> EPVKFKDCGSWVGVIKEVNVSPCPTQPCKLHRGQSYSVNVTFTSNTQSQSSKAVVHGIVMGIPVPFPIPESDGCKSGIRCPIEKDKTYNYVNKLPVKNEYPSIKVVV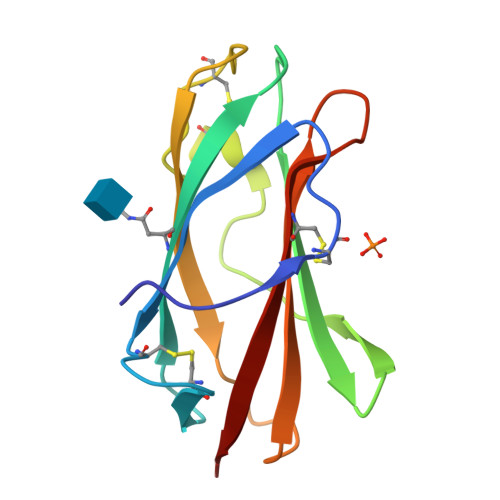EWELTDDKNQRFFCWQIPIEVEA>MTKEPRNLSEWIKELKKASREAVILVEGKNDKKALSKFSIKNVIDLSGKRYADVVDMLEGKWEKVILLF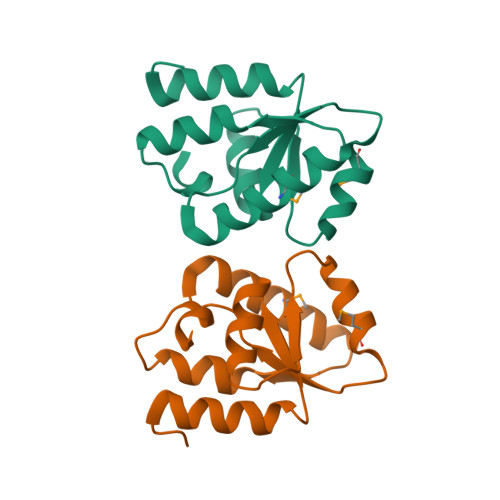DLDTHGERINQKMKELLSSQGFLVDENFRNFLKKWNIIHIEEINGGKNS[2x]>MATNLRGVMAALLTPFDQQQALDKASLRRLVQFNIQQGIDGLYVGGSTGEAFVQSLSEREQVLEIVAEEGKGKIKLIAHVGCVTTAESQQLAASAKRYGFDAVSAVTPFYYPFSFEEHCDHYRAIIDSADGLPMVVYNIPALSGVKLTLDQINTLVTLPGVGALKQTSGDLYQMEQ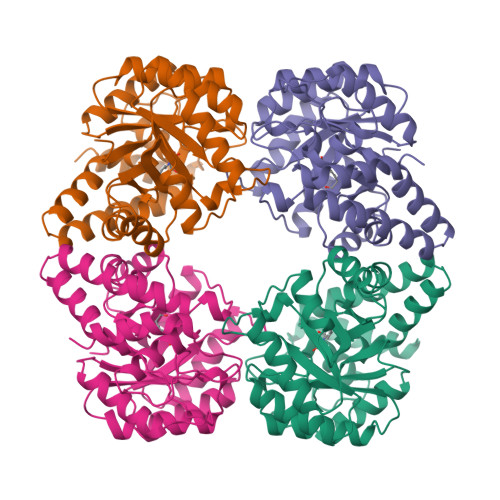IRREHPDLVLYNGYDEIFASGLLAGADGGIGSTYNIMGWRYQGIVKALKEGDIQTAQKLQTECNKVIDLLIKTGVFRGLKTVLHYMDVVSVPLCRKPFGPVDEKYLPELKALAQQLMQERG[4x]> MKKITSVCALLSLICSFNASAEWTGDYENIGYFSHEVISEFHVGQIDGGAYFCIKAVKADGSRSTPLIACSVSNESVWAPSFKVLLEQARYFYVTEQSVRIYYDHNVWTNQPFVNTFSTNAL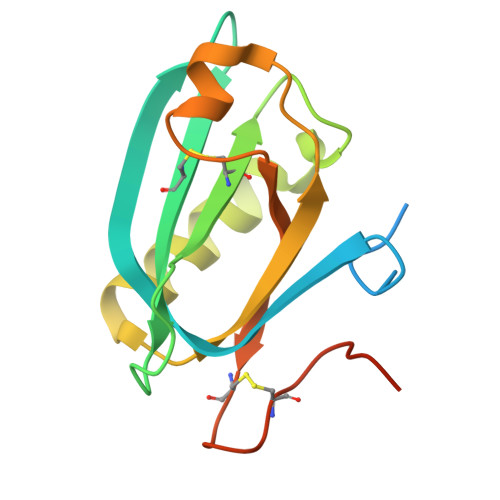VGLSSCSAATDCFGPGKPKSKSKRDVEQ> GDPFGHVASPQSTKRFFIIKSNRMSNIYTSIQHGVWATSKGNSRKLSNAFTSTDHVLLLFSANESGGFQGFGRMMSLPDPQLFPGIWGPVQLRLGSNFRVMWLKQCKIEFEELGKVTNPWNDDLPLRKSRDGTEVPPALGSLL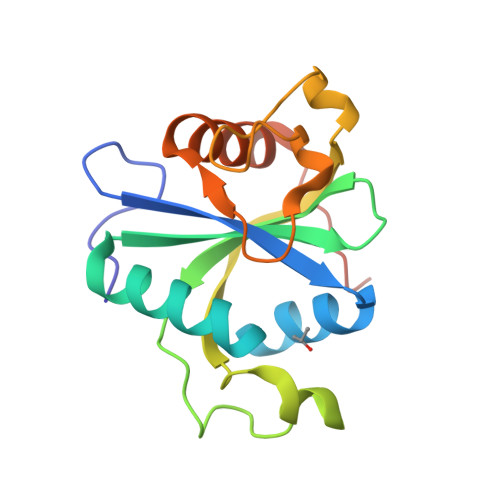CTWMSQRPSEDLLAGTGIDPATR> GPLGSAPVRSLNCTLRDSQQKSLVMSGPYELKALHLQGQDMEQQVVFSMSFVQGEESNDKIPVALGLKEKNLYLSCVLKDDKPTLQLESVDPKNYPKKKMEKRFVFNKIEINNKLEFESAQFPNWYISTSQAENMPVFLGGTKGGQDITDFTMQFVSS;> ADPSERCDDWGLDTMRQIQVFEDEPARIKCPLFEHFLKFNYSTAHSAGLTLIWYWTRQDRDLEEPINFRLPENRISKEKDVLWFRPTLLNDTGNYTCMLRNTTYCSKVAFPLEVVQKDSCFNSPMKLPVHKLYIEYGIQRITCPNVDGYFPSSVKPTITWYMGCYKIQNFNNVIPEGMNLSFLIALISNNGNYTCVVTYPENGRTFHLTRTLTVKVVGSPKNAVPPVIHSPNDHVVYEKEPGEELLIPCTVYFSFLMDSRNEVWWTIDGKKPDDITIDVTINESISHSRTEDETRTQILSIKKVTSEDLKRSYVCHARSAKGEVAKAAKVKQKHHHHHH;> ADPFTLQPAAHTGAARSCRFRGRHYKREFRLEGEPVALRCPQVPYWLWAS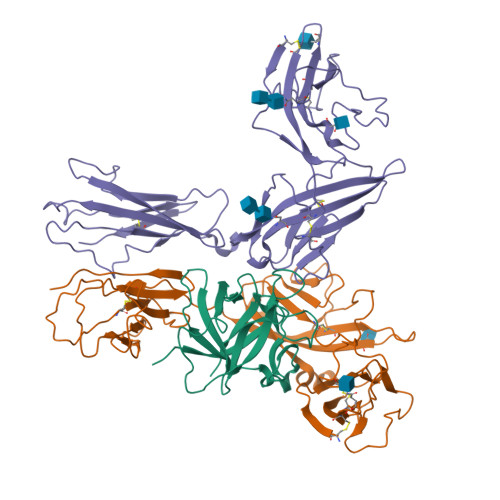VSPRINLTWHKNDSARTVPGEEETRMWAQDGALWLLPALQEDSGTYVCTTRNASYCDKMSIELRVFENTDAFLPFISYPQILTLSTSGVLVCPDLSEFTRDKTDVKIQWYKDSLLLDKDNEKFLSVRGTTHLLVHDVALEDAGYYRCVLTFAHEGQQYNITRSIELRIKKKKEETIPVIISPLKTISASLGSRLTIPCKVFLGTGTPLTTMLWWTANDTHIESAYPGGRVTEGPRQEYSENNENYIEVPLIFDPVTREDLHMDFKCVVHNTLSFQTLRTTVKEHHHHHH>MVKLILVRHAESEWNPVGRYQGLLDPDLSERGKKQAKLLAQELSREHLDVIYSSPL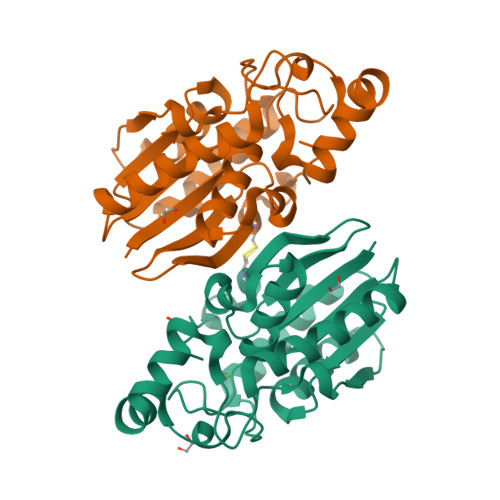KRTYLTALEIAEAKNLEVIKEDRIIEIDHGMWSGMLVEEVMEKYPEDFRRWVEEPHKVEFQGGESLASVYNRVKGFLEEVRKRHWNQTVVVVSHTVPMRAMYCALLGVDLSKFWSFGCDNASYSVIHMEERRNVILKLNITCHLGEFYVEAHKAI[2x]>MGSTKLKGDIAQQAAIMRALKMGWGVLKPLGDRLSYDLVFDVEGILLKVQVKSSWKSEKTGNYVVDNRRT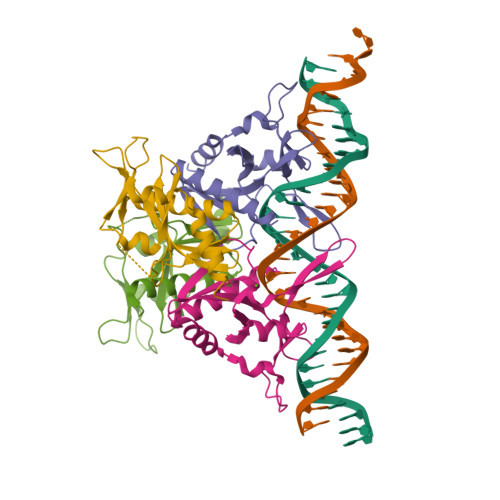RTNRRNIVRSPYRGNDFDFAVAYVEELELFYVFPVDVFISYGSEIHLVETDKRQRKPRSFGYREAWHLILQKGAAQKETSA[4x]> GSGETGEKTPETVALLQNLKQAERKGILFGHHDDTAYGIGWEGDKGRSDVKSVCGAYPGVMSFDLGEIELGGTHNLDKVSFAHLREYIIEQYARGGMISLSWHVRNPKTGGDSWDVTDSTVVASVMQGGENHVKMLEWIDRVADFLLSLKTKEGVLIPVVFRPWHEHTGSWFWWGKDLCSSEQYKTLWRMTNDRLRLKGVNNVLLAYSPGMESDTVEEYLERYPGDDIIDVLGTDVYQFERSQYIKQL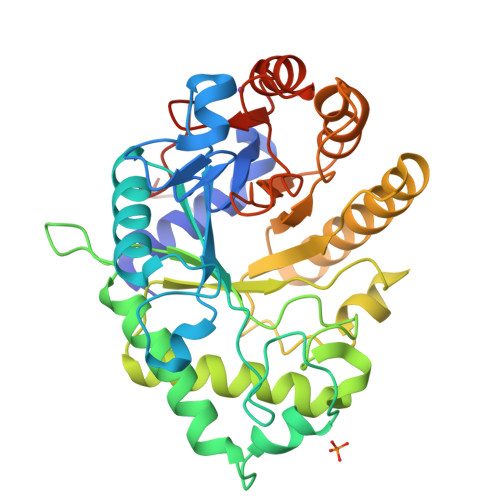NKMLTILTEAGKKHDKPIALTETGLEGIPDSLWWTGTLLPVIEKYPLSYVLVWRNAREKSTHYYAPYPGQVSADDFVKFSRSPKILFVGDNFELYKLEHHHHHH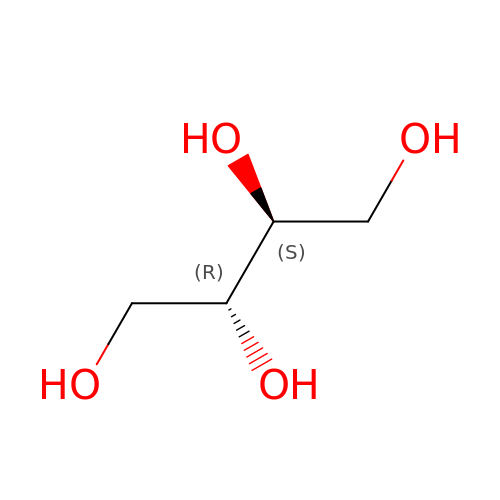MESO-ERYTHRITOL | C4 H10 O4 | UNXHWFMMPAWVPI-ZXZARUISSA-N> METTEVIEGKNITVERTGEENRRLIFQDCLCAVCGLCGEICPVSAIEVNPTGAMVR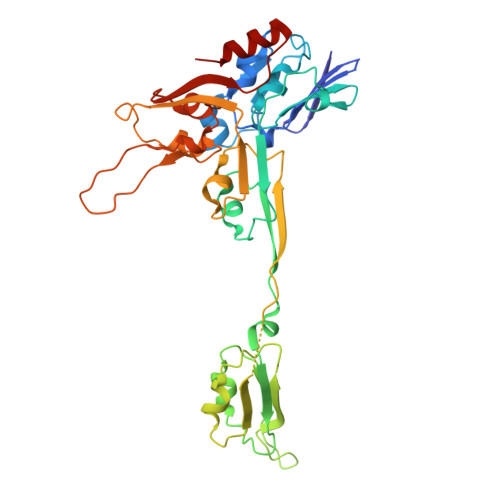TEQEKSKIAIDENKCVLCGMCSSICPFQALDLQIDGTSIKELAEYPKIIKSAEIDDETCIQCKACETACPQDAITITRELPERKDLVTGEIEIDKDTCIYCGMCEEMCPVDAIEIDHQTPSSASPVVATDIRVDEDKCVHCGICKRICPVDAIMQVCRICPYGEYEIKTPEVTGTSYIDPELCVNCGWCQEICPVDAATVTKPFEGELIIDQDTCQACETCVMVCPCNVLSFPKPEKPGEKTTKLHKDERFCIYCGACERSCPVTAITVKRNRINTTPIRSKAWKNAFDSLLK>[3x]MGSSHHHHHHSQDPMFDIKRKTIEWGGKTLVLETGRIARQADGAVLATMGETVVLATAVFAKSQKPGQDFFPLTVNYQEKTFAAGKIPGGFFKREGRPSEKETLVSRLIDRPIRPLFVKGFKNEVQVVVTVLQHDLENDPDILGMVAASAALCLSGAPFMGPIGAARVGWVDGAYVLNPTLDEMKESKMDLVVAGTADAVMMVESEIQELSEEIVLGGVNFAHQQMQAVIDAIIDLAEHAAKEPFAFEPEDTDAIKAKMKDLVGADIAAAYKIQKKQDRYEAVGAAKKKAIAALGLSDENPTGYDPLKLGAIFKELEADVVRRGILDTGLRIDGRDVKTVRPILGEVGILPRTHGSALFTRGETQAIVVATLGTGDDEQFIDALEGTYKESFLLHYNFPPYSVGETGRMGSPGRREIGHGKLAWRALRPMLPTKEDFPYTIRLVSEITESNGSSSMATVCGSSLAMMDAGVP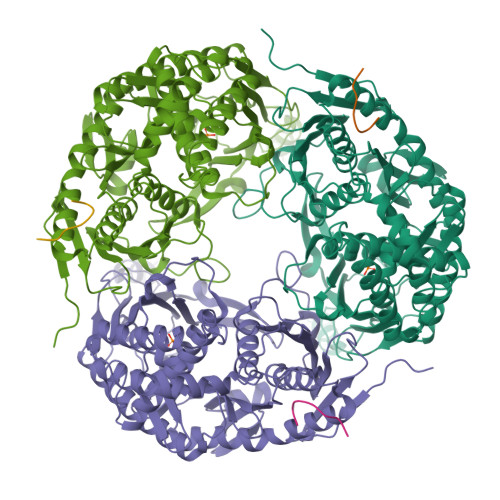LVRPVSGIAMGLILEQDGFAVLSDILGDEDHLGDMDFKVAGTSEGLTSLQMDIKIAGITPAIMEQALAQAKEGRAHILGEMNKAMDAPRADVGDFAPKIETINIPTDKIREVIGSGGKVIREIVATTGAKVDINDDGVVKVSASDGAKIKAAIDWIKSITDEAEVGKIYDGKVVKVVDFGAFVNFFGAKDGLVHVSQISNERVAKPSDVLKEGQMVKVKLLGFDDRGKTKLSMKVVDQETGEDLSKKEAAAEEA;>TAPPEKPRRGWWRR[3x]>[2x]GAGAGAGAGAGMARHFVLNTGAKIPSVGLGTWQSDPGVVGDAVYAAVKAGYRHIDCARVYGNEKEIGLALKKLFEEGVVKR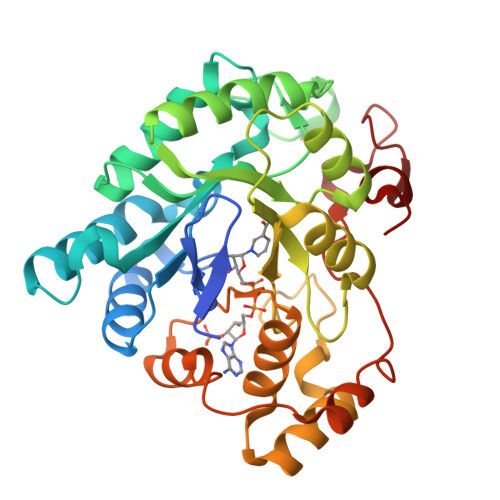EDLFITSKLWNDHHAPEDVPEALNESLKDLQLDYLDLYLIHWPFRVKKGTNTSPENFITPDIPATWGAMEKLYDAGKARAIGVSNFSSKKLGDLLAVARVPPAVDQVECHPGWQQTKLHNFCQSTGVHLSAYSPLGSPGTTWMNGNVLKEPVIISIAEKLGKTPAQVALRWNIQMGHSVLPKSTNEERIKQNLDVYDWSIPDDLLAKFSEIKQARLLRGNFIVNPQSVYKTHEELWDGEL> MTTLADVKKRIGLKDEKQDEQLEEIIKSCESQLLSMLPIEVEQIP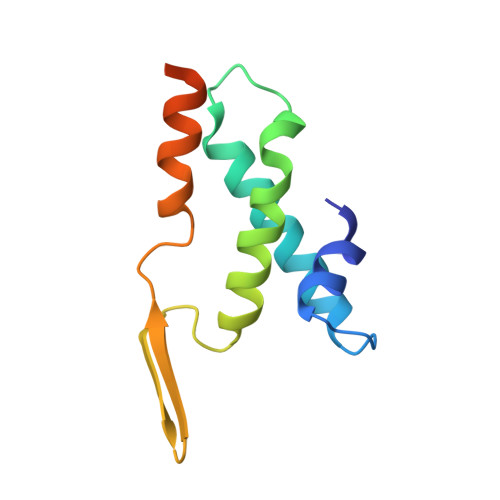ERFSYMIKEVAVKRYNRIGAEGMTSEAVDGRSNAYELNDFKEYEAIIDNYFNARTRTKKGRAVFF>[4x]MSDENNKGVGTAVQGVGGPRDGRTAPGEQGTTLTTRQGHPVHDNQNSRTVGSRGPMTLENYQFIEKLSHFDRERIPERVVHARGVGAHGVFRATGKVGDEP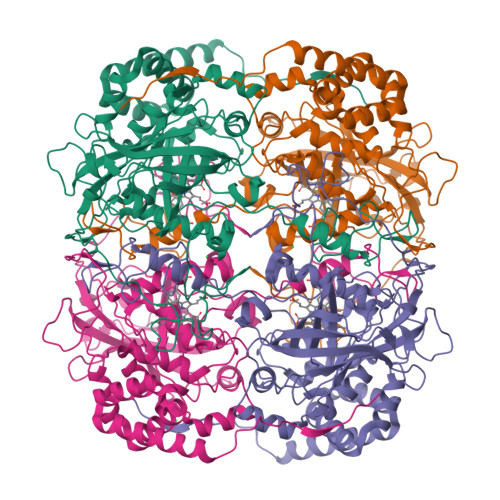VSKYTRAKLFQEDGKETPVFVRFSTVGHGTHSPETLRDPRGFAVKFYTEDGNWDLVGNNLKIFFIRDALKFPDLIHSQKPSPTTNIQSQERIFDFFAGSPEATHMITLLYSPWGIPASYRFMQGSGVNTYKWVNDQGEGVLVKYHWEPVQGVRNLTQMQADEVQATNFNHATQDLHDAIERGDFPQWDLFVQIMEDGEHPELDFDPLDDTKIWPREQFPWRHVGQMTLNRNPENVFAETEQAAFGTGVLVDGLDFSDDKMLQGRTFSYSDTQRYRVGPNYLQLPINAPKKHVATNQRDGQMAYRVDTFEGQDQRVNYEPSLLSGPKEAPRRAPEHTPRVEGNLVRAAIERPNPFGQAGMQYRNFADWERDELVSNLSGALAGVDKRIQDKMLEYFTAADADYGQRVREGIQAKEAEMKGQKQEAPVYGTEASSLY> MTGPVNPDDRRSFSSRTPVNENPDGVQYRRGFVTRHQVSGWRFVMRRIASGVALHDTRMLVDPLRTQSRAVLTGALILVTGLVGCFIFSLFRPGGVPGNNAILADRSTSALYVRVGEQLHPVLNLTSARLISGSPDNPTMVKTSEIDKFPRGNLLGIPGAPERMVQNAATDAEWTVCDAVGGANPGVTVIAGPLGADGERAAPLPPDHAVLVHSDAEPNPGDWLLWDGKRSPIDLADRAVTDALGLGGQAL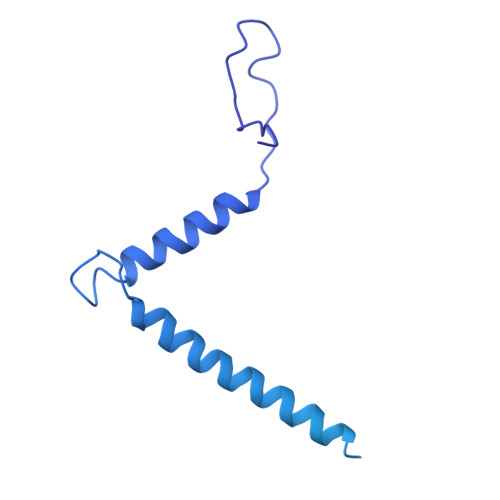APRPIAAGLFNAVPAAPALTAPVIPDAGAAPQFELSLPVPVGAVVVAYDADNTARYYAVLSDGLQPISPVLAAILRNTDSHGFAQPPRLGPDEVARTPMSRGLDTSAYPDNPVTLVEASAHPVTCAHWTKPSDAAESSLSVLSGAVLPLAEGLHTVDLVGAGAGGAANRVALTPGTGYFVQTVGAEPGSPTAGSMFWVSDTGVRYGIDTAEDDKVVAALGLSTSPLPVPWSVLSQFAAGPALSRGDALVAHDAVSTNPNSARMEASR GEMCITABINE | C9 H11 F2 N3 O4 | 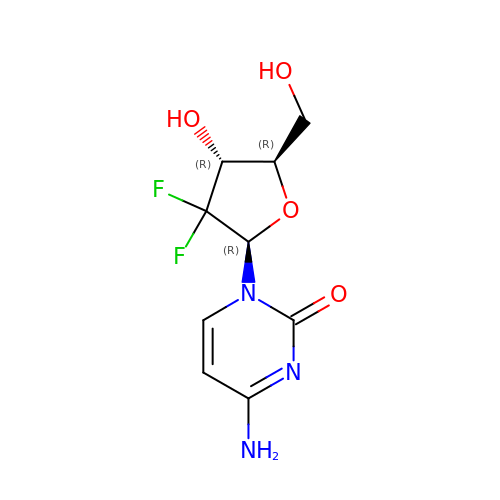SDUQYLNIPVEERB-QPPQHZFASA-N2-({[3-FLUORO-3'-(TRIFLUOROMETHOXY)BIPHENYL-4-YL]AMINO}CARBONYL)CYCLOPENT-1-ENE-1-CARBOXYLIC ACID | C20 H15 F4 N O4 | 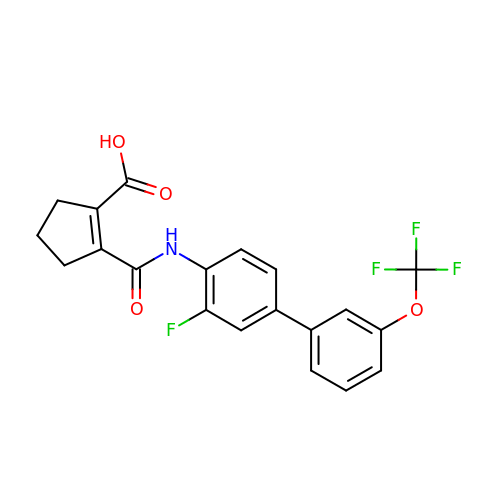CTKBCQCRHRCICI-UHFFFAOYSA-N>GSMSLPDGFYIRRMEEGDLEQVTETLKVLTTVGTITPESFCKLIKYWNEATVWNDNEDKKIMQYNPMVIVDKRTETVAATGNIIIERKIIHELGLCGHIEDIAVNSKYQGQGLGKLLIDQLVTIGFDYGCYKIILDCDEKNVKFYEKCGFSNAGVEMQIRK[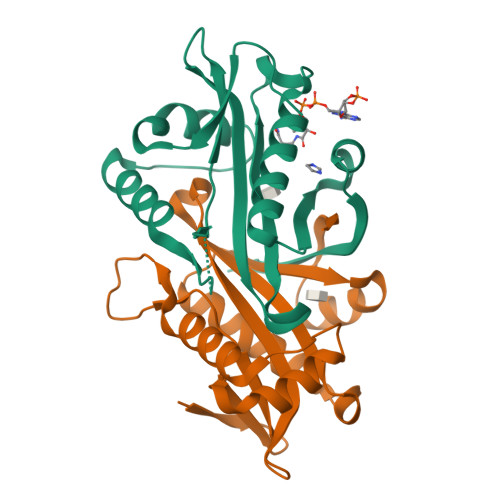4x]>[4x]PFVELETNLPASRIPAGLENRLCAATATILDKPEDRVSV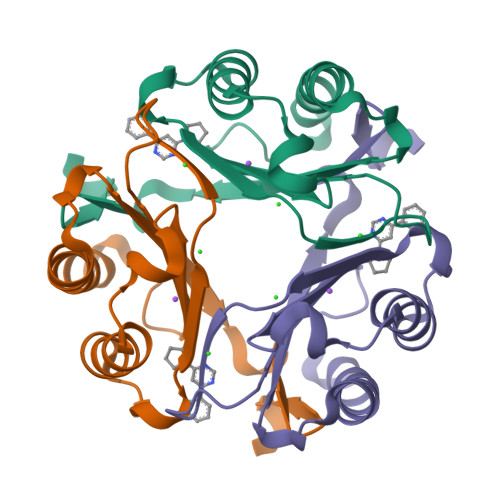TIRPGMTLLMNKSTEPCAHLLVSSIGVVGTAEQNRTHSASFFKFLTEELSLDQDRIVIRFFPLEAWQIGKKGTVMTFL> ANSR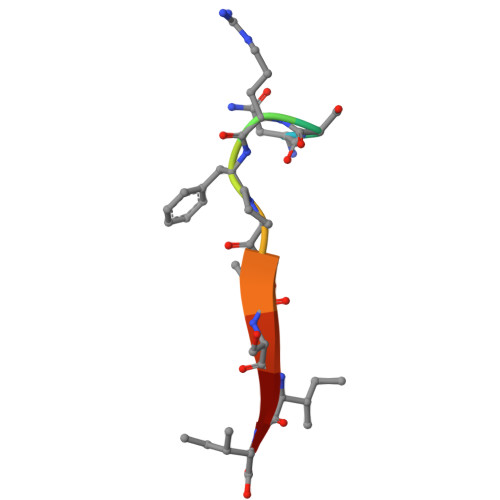FPTSII> AAVTQSPRNK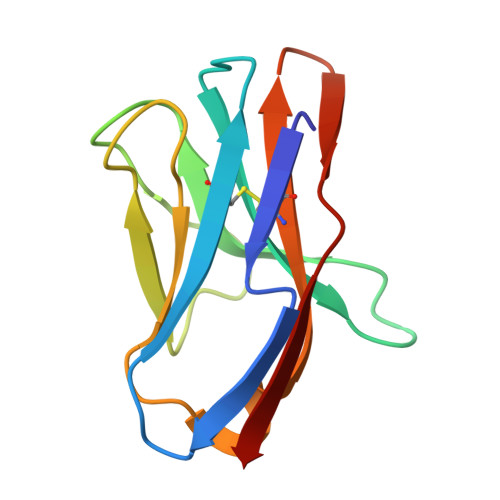VAVTGEKVTLSCQQTNNHNNMYWYRQDTGHGLRLIHYSYGAGSTEKGDIPDGYKASRPSQEQFSLILESATPSQTSVYFCASGGGGTLYFGAGTRLSVL> MGHMNITDIREQFPILHQQVNGHDLVYLDSAATSQKPRAVIETLDKYYNQYNSNVHRGVHT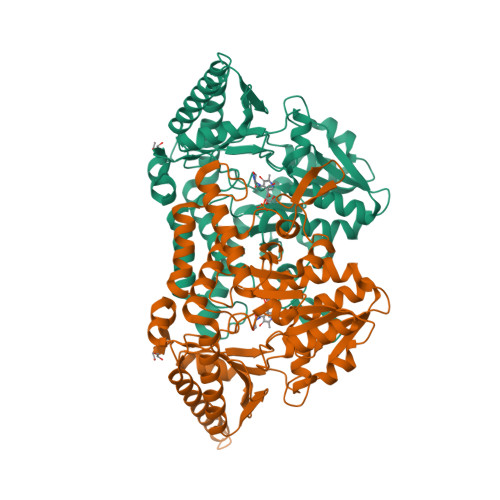LGTRATDGYEGAREKVRKFINAKSMAEIIFTKGTTTSLNMVALSYARANLKPGDEVVITYMEAHANIIPWQQAVKATGATLKYIPLQEDGTISLEDVRETVTSNTKIVAVSHVSNVLGTVNPIKEMAKIAHDNGAVIVVDGAQSTPHMKIDVQDLDCDFFALSSHKMCGPTGVGVLYGKKALLENMEPAEFGGEMIDFVGLYESTWKELPWKFEAGTPIIAGAIGLGAAIDFLEEIGLDEISRHEHKLAAYALERFRQLDGVTVYGPEERAGLVTFNLDDVHPHDVATVLDAEGIAVRAGHHCAQPLMKWLDVTATARASFYLYNTEEEIDKLVEALQKTKEYFTNVFVDLEHHHHHH>[2x]ARKCSLTGKWTNDLGSNMTIGAVNSRGEFTGTYTTAVTATSNEIKESPLHG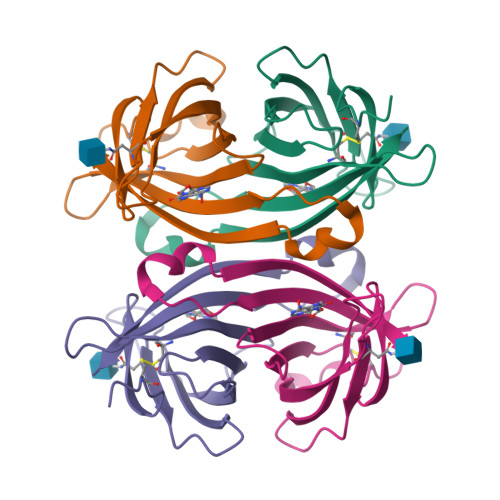TENTINKRTQPTFGFTVNWKFSESTTVFTGQCFIDRNGKEVLKTMWLLRSSVNDIGDDWKATRVGINIFTRL>[3x]GPLGSDNKVLHVYNWSDYIAPDTLEKFTKETGIKVVYDVYDSNEVLEAKLLAGKSG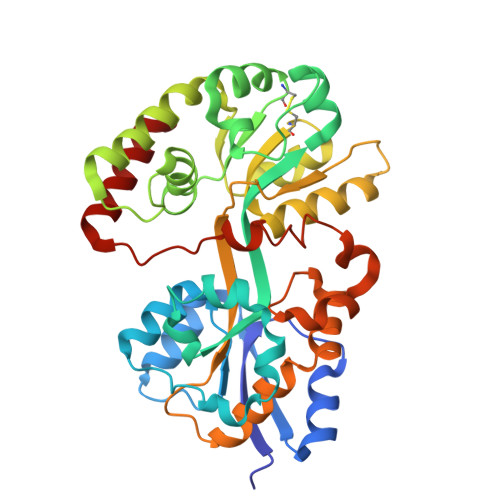YDVVVPSNSFLAKQIKAGVYQKLDKSKLPNWKNLNKDLMHTLEVSDPGNEHAIPYMWGTIGIGYNPDKVKAAFGDNAPVDSWDLVFKPENIQKLKQCGVSFLDSPTEILPAALHYLGYKPDTDNPKELKAAEELFLKIRPYVTYFHSSKYISDLANGNICVAIGYSGDIYQAKSRAEEAKNKVTVKYNIPKEGAGSFFDMVAIPKDAENTEGALAFVNFLMKPEIMAEITDVVQFPNGNAAATPLVSEAIRNDPGIYPSEEVMKKLYTFPDLPAKTQRAMTRSWTKIKS>MKPHALIGLLAGMLLSSSLYAADSTKPLPLHIGGRVLVESPANQPVSYTYSWPAVYFETAFKGQSLTLKFDDDQNIFRLIVDDKAPVVINKPGKVDYPVESLAPGKHRVRLEKLTETQSTSGRFLGFYTDPSAKPLALPKRKRQIEFIGDSFTVGYGNTSPSRECTDEELFKTTNSQMAFGPLTAKAFDADYQINASSGFGIVRNYNGTSPDKSLLSLYPYTLNNPDQLYHNKHWKPQVIVIGLGTNDFSTALNDNERWKTREALHADYVANYVKFVKQLHSNNARAQFILMNSDQSNGEIAEQVGKVVAQLKGGGLHQVEQIVFKGLDYSGCHWHPSANDDQLLANLLITHLQQKKGIWLEHHHH[2x]

CE2 enzymes are acetyl esterases (that are generally not appended to other catalytic modules), which are reported to be active on synthetic aryl-esters and acetylated xylan. Here we report the biochemical properties and crystal structure of several CE2 members, both single-module CE2 enzymes and CtCE2, a component of CtCel5C-CE2. All three 3D structures reveal a bi-domain enzyme in which an N-terminal β-sheet “jelly roll” domain (around 130 residues) is linked to a C-terminal domain of approximately 220 residues. The C-terminal domains possess an atypical α/β-hydrolase (SGNH-hydrolase) fold, consisting of repeating β-α-β motifs that form a curved central five-stranded parallel β-sheet, in the strand order β2, β1, β3, β4, and β5 with strand β2 interrupted by loop insertion.

CtCE2 along with CjCE2B does not possess a side-chain residue equivalent to the Asp of a classical Ser-His-Asp triad. Instead, these enzymes display a catalytic dyad with stabilisation of the histidine provided by main-chain carbonyl groups. Instead of the more typical Ser-His-Asp, the “triad” geometry is completed through the Nɛ1 of His-791 making a hydrogen bond with the backbone carbonyl of Glu-788, in the case of CtCE2, whilst the equivalent interaction in CjCE2B is with the main-chain carbonyl of Cys-333. Based on their catalytic efficiencies, CtCE2 and CjCE2B exhibit a significant preference for acetylated glucomannan over xylan, whereas CjCE2A and CjCE2C do not distinguish between the two polysaccharides. Pull-down assays revealed that none of the Cellvibrio enzymes bound to insoluble cellulose. While the binding of CjCE2A or CjCE2C to polysaccharides could not be detected by ITC (unpublished data) or AGE, CjCE2B interacted with, β-glucan, albeit with ∼17-fold lower affinity than CtCE2, but did not recognize carboxymethylcellulose (unpublished data) or hydroxyethylcellulose. Although the two structurally characterised Cellvibrio esterases do not bind cellohexaose or cellulose, they do contain aromatic residues in the cleft that houses the active site. Thus, Tyr-665 in CtCE2 is conserved in the C. japonicus esterases (Trp-231 in CjCE2A and Tyr-206 in CjCE2B), while Trp-335 in CjCE2B is equivalent to Trp-790 in the Clostridium enzyme.> MDVAGLTDCGLIRKSNQDAFYIDEKHQRFFIVADGMGGHAGGEEASRLAVDHIRQYLETHLEDLQHDPVTLLRQAFLAANHAIVEQQRQNSARADMGTTAVVILLDEKGDRAWCAHVGDSRIYRWRKDQLQQITSDHTWIAQAVQLGSLTIEQARQHPWRHVLSQCLGREDLSQIDIQPIDLEPGDRLLLCSDGLTEELTDDVISIYLSEPNVQKAAAALVDAAKTHGGRDNVTVVV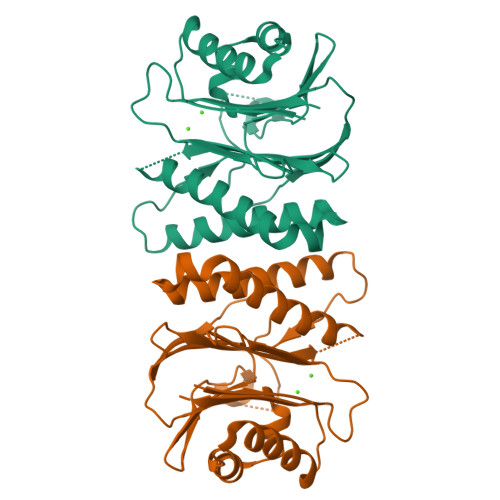ISV> HHMSAIKPDMKINLRMEGNVNGHHFV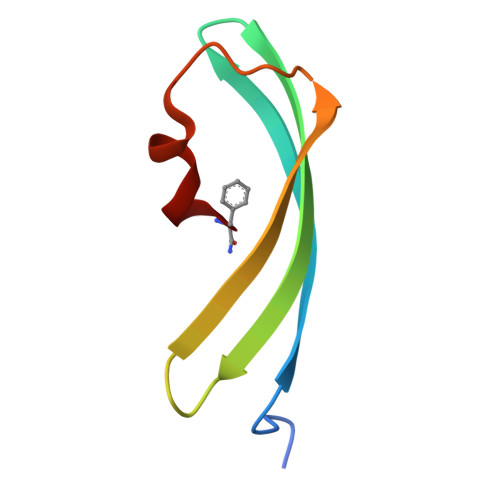IDGDGTGKPFEGKQSMDLEVKEGGPLPFAFDILTTAF[1-(2-oxoethyl)-1H-1,2,3-triazol-5-yl]methyl 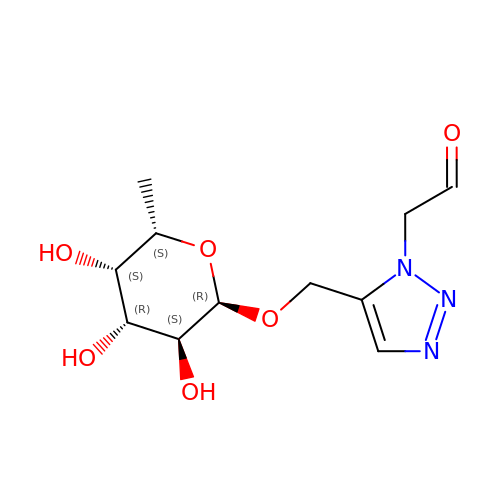6-deoxy-alpha-L-galactopyranoside | C11 H17 N3 O6 | VXMWUAUJLLGYLQ-GDWDKGMLSA-N5-(4-fluorophenyl)-2,3-dihydroxy-N-(2-hydroxyethyl)benzamide | C15 H14 F N O4 | 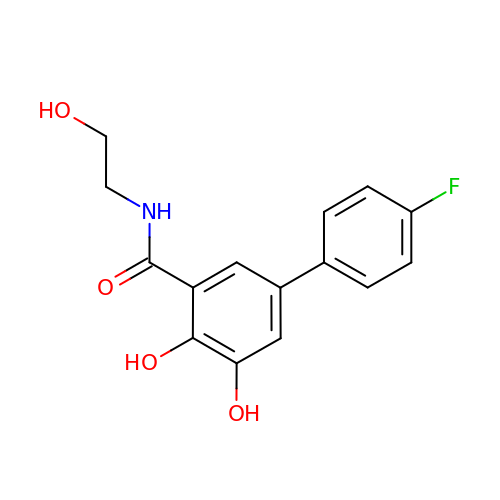ASGZSLFHJDBZNV-UHFFFAOYSA-N>[2x]GMEVNQPDIVAQ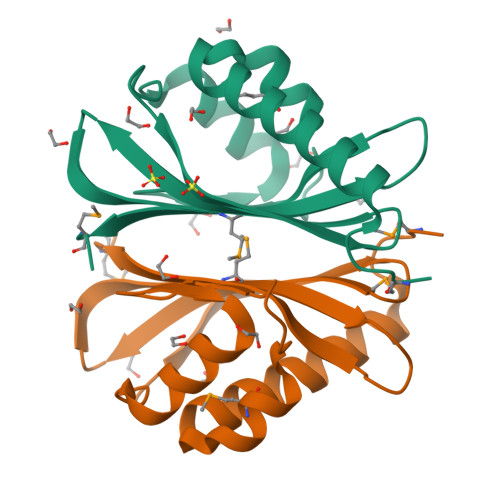VQAAFVEYERALVENDIEAMNALFWHTPETVRYGIAEVQHGGEAIRAWRERCEPVPKSRKLHRTVVTTFGTDFATVSTEFTSDATPLLGRQMQTWARLSPADGWKIVAAHVSLIAMP CLKs are dual-specificity kinases that are activated by autophosphorylating their own tyrosine residues and subsequently phosphorylate the serine/threonine residues of the SR protein. Later, CX-4945 was revealed to have a strong inhibitory activity on CLKs; IC50 values of 82.3 nM (CLK1), 3.8 nM (CLK2), and 90.0 nM (CLK3). In order to elucidate the selective inhibitory effect of CX-4945 on CLKs, we determined the structures of CLK1, CLK2, and CLK3 in complex with CX-4945. The overall structure of the CLK catalytic domain contained 12 β-strands and 10 α-helices that could be divided into the N-lobe and C-lobe, which are typical forms of the kinase.

The active site environment of CLK3/CX-4945 was also similar to that of CLK2/CX-4945 except for the valine residue (corresponding to Val324 and Val326 in CLK1 and CLK2, respectively), which was replaced with the Ala319 residue. This substitution may contribute to weaker hydrophobic interactions (see below). The results are consistent with the findings of previous studies showing that CX-4945 more strongly inhibits CLK2 than CLK3. In contrast, CLK3 did not have the entire β-hairpin insertion structure due to its flexibility. CLK3 had the longest C-terminus with an extra seven residues compared with the C-terminus of CLK1. CLK1 had the smallest and CLK3 had the largest pocket size. As described in the previous section, the hydrophobic valine residue (Val324 and Val326 in CLK1 and CLK2, respectively) was substituted with alanine (Ala319) in CLK3. This substitution could result in the weaker hydrophobic interactions compared with the interactions of CLK1 and CLK2.

> MHHCKRYRSPEPDPYLSYRWKRRRSYSREHEGRLRYPSRREPPPRRSRSRSHDRLPYQRRYRERRDSDTYRCEERSPSFGEDYYGPSRSRHRRRSRERGPYRTRKHAHHCHKRRTRSCSSASSRSQQSSKRSSRSVEDDKEGHLVCRIGDWLQEDYEIVGNLGEGTFGKVVECLDHARGKSQVALKIIRNVGKYREAARLEINVLKKIKEKDKENKFLCVLMSDWFNFHGHMCIAFELLGKNTFEFLKENNFQPYPLPHVRHMAYQLCHALRFLHENQLTHTDLKPENILFVNSEFETLYNEHKSCEEKSVKNTSIRVADFGSATFDHEHHTTIVATRHYRPPEVILELGWAQPCDVWSIGCILFEYYRGFTLFQTHENREHLVMMEKILGPIPSHMIHRTRKQKYFYKGGLVWDENSSDGRYVKENCKPLKSYMLQDSLEHVQLFDLMRRMLEFDPAQRITLAEALLHPFFAGLTPEERSFHTSRNPSR>[2x]GSWSGGSGGEAADEARRAIEAALEEARAAADEARSDSTGETVKKAVDKAEKAAEDAFREIKQAVNQAEKQGASEAAFEAFAAIAAAAAEAAAAAFEAFSDSTGETVAEAVAKALKAAMEAFAEIAKAVAQAAKQGASEAAFEAFAAIAAAAAEAAAAAFEAFSDSTGETVAEAVAKALKAAMEAFAEIAKAVAQAAKQGASEAAFEAFAAIAAAAAEAAAAAFEAFSDSTGETVAEAVAKALKAAMEAFAEIAKAVAQAAKQGASEAAFEAFAAIAAAAAEAAAAAFEAFSDSTGETVAEAVAKALKAAMEAFAEIAKAVAQAAKQGASEEAFEKFAAIAAEAAEAAAAAFERFSDSTGETEAEKVAKELKQLMEEFAERAKSVAEQAKNGAS

To test this hypothesis, we design helical repeat proteins (DHRs) displaying regularly spaced carboxylate arrays on their surfaces and find that both protein monomers and protein-Ca2+ supramolecular assemblies directly nucleate nano-calcite with non-natural {110} or {202} faces while vaterite, which forms first in the absence of the proteins, is bypassed. To enable exploration of the contribution of the size of the protein-mineral interface while keeping the chemical composition and geometry otherwise constant, we employed Designed Helical Repeat (DHR)39 proteins that can be shrunk or extended simply by changing the number of repeating units. In contrast to typically designed protein surfaces containing a mix of positive, negative, and non-charged hydrophilic residues to promote solubility, and to hydrophobic protein surfaces designed to bind other proteins, we designed surfaces consisting entirely of carboxylate side chains spaced at regular intervals to mimic the carbonate sublattice on different crystallographic planes of CaCO3 crystals (see “Methods”). Here, we describe the design of DHR proteins that template growth of CaCO3 crystals.

Flat repeat helix-turn-helix-turn protein backbones were designed with either constrained monte-carlo fragment assembly with RosettaRemodel40, or by placing α-helices in a plane and then connecting them with additional secondary structural elements. Two designs, FD15 and FD31, which were monodisperse in size exclusion chromatography experiments (SEC) were selected for detailed characterization. Circular dichroism (CD) experiments showed the expected alpha-helical structure, and the proteins were found to be hyperstable, remaining folded at temperatures up to 95 °C. The crystal structure of FD15 was solved at 4 Å resolution and matched the design model with an RMSD of 0.45 Å with a perfectly straight repeating structure having a 8.7 Å spacing between helices in adjacent repeat subunits. In contrast, FD15 did not alter the crystallization pathway from that seen with the no protein and BSA controls. In contrast, in the presence of (j) FD15 or a BSA control (j) only vaterite is formed (k, l). We found that the spacing of the designed sidechain arrays with similar chemistry had a pronounced effect: FD15 with an array spacing of 0.9 nm did not template calcite, DHR49-Neg with a spacing of 1.0 nm templated calcite to some extent, and FD31 with a 1.1 nm spacing was a strong nucleator of calcite.>MKQGGQGLQDYYLNQLRKEKILATVFLTNGFQLRGRVVSFDNFTVLLDVEGKQQLVFKHAISTFSPQKNVAL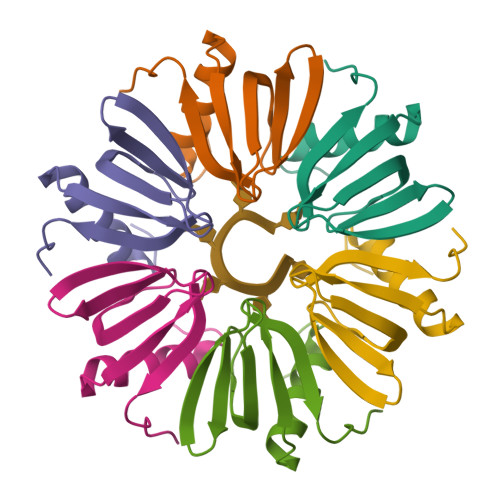NPDAE[12x]> GNSEEDYPNGTWLGDENNPEMRVRCAIIPSDMLHISTNCRTAEKMALTLLDYLFHREVQAVSNLSGQGKHGKKQLDPLTIYGIRCHLFYKFGITESDWYRIKQSIDSKCRTAWRRKQRGQSLAVKSFSRRTPNSSSYCPSE

pmcThe BEN (BANP, E5R, and NAC1) domain is a ∼100-residue protein domain found in metazoans and viruses, but missing in nematodes and urochordates. There are nine BEN domain–containing transcription factors in the human genome, i.e., BANP, BEND2-7, and NAC1/2. The BEN domain-containing transcription factors regulate transcription by recruiting chromatin-modifying factors to specific chromatin regions via their DNA-binding BEN domains. Further structural analysis revealed that although all these BEN domains bind their target DNAs mainly through the insertion of the C-terminal α5 helix into the major groove of DNA, the residues of the α5 helices involved in the base interactions vary from one to another, explaining why they exhibit distinct DNA sequence preference.

We then synthesized a 12-mer DNA fragment with a palindromic sequence of CTCTCGCGAGAG for the crystallization study. We first measured its binding ability to the human BANP BEN domain by ITC, which showed that the BEN domain of BANP bound to the palindromic 12-mer DNA with a Kd of 8.4 μM. In the BANP-DNA complex structure, the extra C-terminal region after the helix α5 in the longer construct is disordered and unresolved in the structure. In the DNA-bound structure, the DNA binding surface of the BANP BEN domain was largely positively charged, which conferred electrostatic interactions with the DNA. The BANP BEN domain interacted with the palindromic DNA mainly through its C-terminal α5 helix, which inserted into the major groove of DNA. Specifically, the side chain of S313 from the α5 helix formed a hydrogen bond with the base of T4, and the side chain of R316 formed two hydrogen bonds with the base of G5′ that is the second G of the CGCG motif. S313 and T317 also formed two water-mediated hydrogen bonds with the base of C3. In addition to these base-engaged interactions, S310, D312, K314, R320, and Q323 from the α5 helix and N269, S271, Q273, and K278 from the loop connecting α3 and α4 (called Loop 1 thereafter) formed several hydrogen bonds or salt bridges with the backbone of DNA. The results showed that mutating N269, S313, R316, and R320 of BANP to alanine individually reduced its DNA binding affinity by ∼2-5-fold compared to the WT BANP. Taken together, our structural and biochemical data demonstrate that the BANP BEN domain mainly utilized the electrostatic interactions to bind DNA with some base-specific interactions with the TC motifs by the α5 helix and Loop 1 of BANP.>MRHPLVMGNWKLNGSRHMVHELVSNLRKELAGVAGCAVAIAPP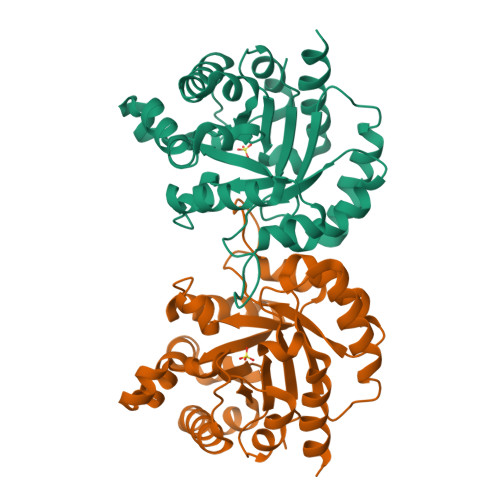EMYIDMAKREAEGSHIMLGAQNVDLNLSGAFTGETSAAMLKDIGAQYIIIGHSERRTYHKESDELIAKKFAVLKEQGLTPVLCIGETEAENEAGKTEEVCARQIDAVLKTQGAAAFEGAVIAYEPVWAIGTGKSATPAQAQAVHKFIRDHIAKVDANIAEQVIIQYGGSVNASNAAELFAQHDVDGFLVGGASLKPEFVDIINAAEAAKQA[4x]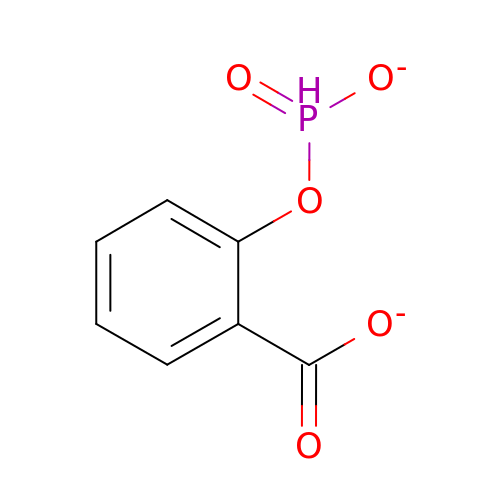2-[(DIOXIDOPHOSPHINO)OXY]BENZOATE | C7 H5 O5 P | BTPFLIXGJHTRNG-UHFFFAOYSA-L4-{6-(tert-butylsulfonyl)-7-[2-(4-methylpiperazin-1-yl)ethoxy]imidazo[1,2-a]pyridin-3-yl}-6-chloropyridin-2-amine | C23 H31 Cl N6 O3 S | 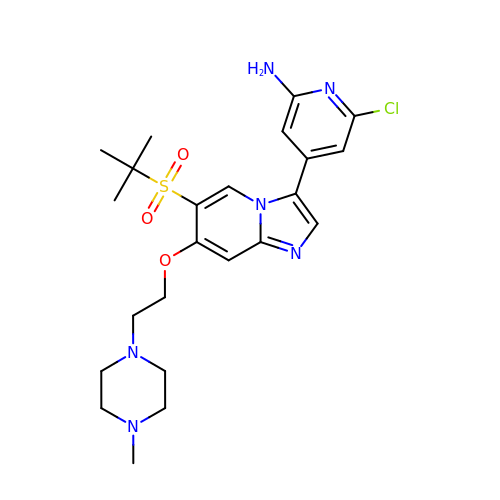PIIVPMZRLRQOTG-UHFFFAOYSA-N>[12x]EDPHLRNRPGKGHNYIDGMTQEDATCKPVTYAGACSSFDVLLEKGKFPLFQSYAHHRTLLEAVHDTIIAKADPPSCDLQSAHGNPCMKEKLVMKTHCPNDYQSAHYLNNDGKMASVKCPPKYELTEDCNFCRQMTGASLKKGSYPLQDLFCQSSEDDGSKLKTKMKGVCEVGVQALKKCDGQLSTAHEVVPFAVFKNSKKVYLDKL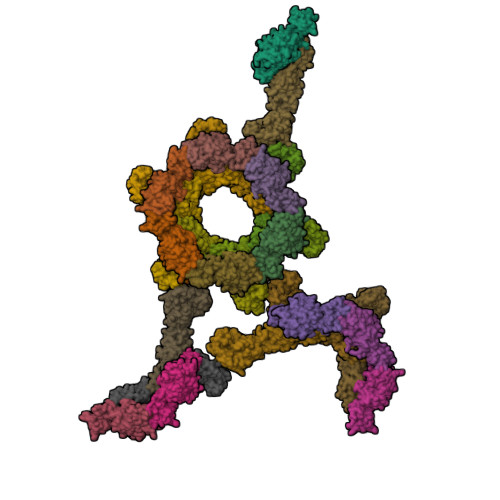DLKTEENLLPDSFVCFEHKGQYKGKLDSGQTKRELKSFDISQCPKIGGHGSKKCTGDAAFCSAYECTAQYANAYCSHANGSGIVQIQVSGVWKKPLCVGYERVVVKRELS;>DPGCSELIQASSRITTCSTEGVNTKCRLSGTALIRAGSVGAEACLMLKGVKEDQTKFLKIKTVSSELSCREGQSYWTGSFSPKCLSSRRCHLVGECHVNRCLSWRDNETSAEFSFVGESTTMRENKCFEQCGGWGCGCFNVNPSCLFVHTYLQSVRKEALRVFNCIDWVHKLTLEITDFDGSVSTIDLGASSSRFTNWGSVSLSLDAEGISGSNSFSFIESPGKGYAIVDEPFSEIPRQGFLGEIRCNSESSVLSAHESCLRAPNLISYKPMIDQLECTTNLIDPFVVFERGSLPQTRNDKTFAASKGNRGVQAFSKGSVQADLTLMFDNFEVDFVGAAVSCDAAFLNLTGCYSCNAGARVCLSITSTGTGSLSAHNKDGSLHIVLPSENGTKDQCQILHFTVPEVEEEFMYSCDGDERPLLVKGTLIAID[12x]>[8x]MHHHHHHAMGTKKSAAEASKKPRQKRTATKQYNVTQAFGRRGPEQTQGNFGDQDLIRQGTDYKHWPQIAQ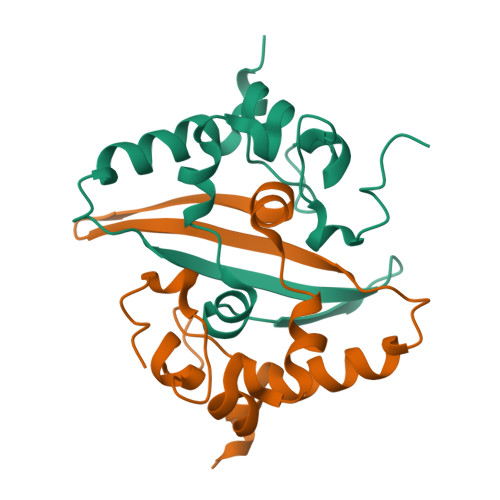FAPSASAFFGMSRIGMEVTPSGTWLTYHGAIKLDDKDPQFKDNVILLNKHIDAYKTFP> DQFSPECSAVTHIFQARGIDAIEIPQKPSNERVLRYCESPSVGTCCTYNMETRMAMQSRQQLEGHTKDQISRMSGILGSKATKFKDIFTALLKESR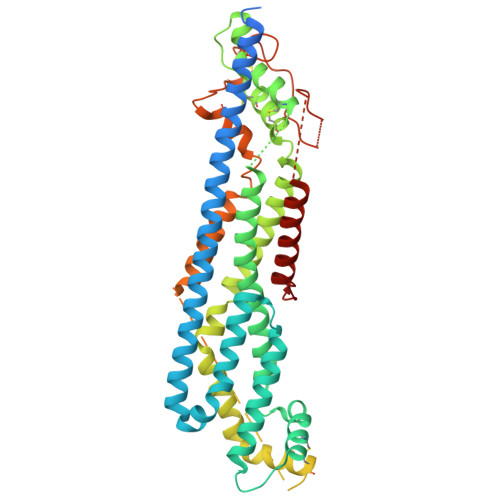TQFNSMFIRTYGVIYERNSYVFSDLFKELETYFANGRVDLLEVMDKFFNTLYQKMFTVLNTQYTFDENYMRCVSEHMKELKPFGDVPDKLSVQIKRSFVATRTYGQALTTASEVAKKVLNVRLNADCTGALTKMQHCGACKGYTEKPCTNYCVNVIKGCLHYQHEFDSEWENFAMAMDKVAERLLGSFNIVMVVEPLNIKISEAIMNFQDSGQDITNRVFQGCGRPKLKKRERRAAEPGSQETSSQQSQEQGVGKSGNGGGGGGGNNRRQQQRRKQQQQRRKQQNNRDDNDDDDEESGGGREPILDRIVRDIRQRVKDYKKFWSNLPHSVCSNEDIASSSDVDGMCWNGHTIDRYMHSITTEHGSNPEFTGNPASTKQTAQMASQLSHLKNAIVHLRNAYNGQDVEWSEQ GlgE is an α-maltose 1-phosphate:(1→4)-α-d-glucan 4-α-d-maltosyltransferase (starch synthase (maltosyl-transferring), EC 2.4.99.16) and a member of the carbohydrate-active enzymes database (CAZy) GH13_3 family. It is the third and defining enzyme of the four-step GlgE pathway that is responsible for the biosynthesis of a branched α-glucan. The key contribution that GlgE makes is to preferentially extend A chains, limiting the opportunity for GlgB to introduce a second branch into B and C chains. The enzyme consists of five domains, four of which are typical of the α-amylase family.

In an attempt to obtain a structure of a trapped maltosyl-enzyme intermediate with an acceptor bound in a productive conformation, we soaked a crystal of the E423A variant of GlgE in both malto-octaose and 2-deoxy-2-fluoro-α-maltosyl fluoride. Fortuitously, this yielded a structure where malto-octaose was bound such that it occupied both the donor and cyclodextrin binding sites, whereas the donor analogue was unexpectedly absent from the crystal. This structure would therefore appear to represent a product-bound species with subsites −2 to +6 occupied. The two sugar residues in the donor site are oriented in a manner similar to those observed with maltose and α-maltose 1-phosphate. The residues occupying subsites +3 to +6 overlap with those seen in cyclodextrins and the maltopentaose described above but are somewhat displaced to allow the product to bind in the appropriate orientation. The conformation of the oligosaccharide was unusually flat and extended compared with amylose or amylopectin, which have α-1,4 torsion angles closer to that of maltose (ϕ = 116° and ψ = −118°). This was particularly striking at the linkage where the donor and acceptor glucose residues occupying subsites −1 and +1 connect (ϕ = 34° and ψ = −157°), giving the longest distance between the 2- and 3′-hydroxyl oxygens of 4.9 Å. The product-bound structures of the E423A variant of GlgE had an additional malto-oligosaccharide bound at a secondary site located on domain C. In each case, five glucose residues were well resolved, clearly showing that they that were wrapped around Tyr-646 of S. coelicolor GlgE.

>MGSSHHHHHHSSGLVPRGSHMPATHHSSATSAERPTVVGRIPVLDVRPVVQRGRRPAKAVTGESFEVSATVFREGHDAVGANVVLRDPRGRPGPWTPMRELAPGTDRWGATVTAGETGTWSYTVEAWGDPVTTWRHHARIKIPAGLDTDLVLEEGARLYERAAADVPGREDRRELLAAVDALRDESRPAASRLAAALTPQVDAVLARHPLRDLVTSSDPLPLLVERERALYGAWYEFFPRSEGTPHTPHGTFRTAARRLPAIAAMGFDVVYLPPIHPIGTTHRKGRNNTLSATGDDVGVPWAIGSPEGGHDSIHPALGTLDDFDHFVTEAGKLGLEIALDFALQCSPDHPWVHKHPEWFHHRPDGTIAHAENPPKKYQDIYPIAFDADPDGLATETVRILRHWMDHGVRIFRVDNPHTKPVAFWERVIADINGTDPDVIFLAAAFTRPAMMATLAQIGFQQSYTYFTWRNTKQELTEYLTELSGEAASYMRPNFFANTPDILHAYLQHGGRPAFEVRAVLAATLSPTWGIYSGYELCENTPLREGSEEYLDSEKYQLKPRDWTRAAREGTTIAPLVTRLNTIRRENPALRQLRDLHFHPTDKEEVIAYSKRQGSNTVLVVVNLDPRHTQEATVSLDMPQLGLDWHESVPVRDELTGETYHWGRANYVRLEPGRTPAHVCTVLRPSHPQIGGSHTT[2x]>MATLKAQHLAKSYKGRQVVRDVSMSIDSGQIVGLLGPNGAGKTTCFYMIVGLVQADQGVVRIDEQNVTHLPMHGRARAGIGYLPQEASIFRKLSVSDNIMAILETRSDLDRNGRKEALEGLLQEFHIHHIRDNLGMSLSGGERRRVEIARALASAPKFILLDEPFAGVDPISVGDIKQIIHHLKAKGIGILITDHNVRETLDICETAYIVNDGQLIAEGDAESILANDLVKEVYLGHEFRLHHHHHH[2x];> MIVFRYLSREVLVTMSAVSAVLLVIIMSGRFIKYLAQAAQGLLDPGSLFLIMAFRIPGFLQLILPLGLFLGILLAYGRLYLESEMTVLSATGMSQKRLLGYTMAPALLVAILVAWLSLFLAPQGINQFALLLNKQDTLTEFDTLVPGRFQAMRDGTRVTYTEELSKDRGELAGIFISQKDLNSSNQERGISILVAEKGTQNIQADGSRYLILHNGYRYDGNPGQANYRAIQYDTYGVMLPKPEASSEVSERDAVPTADLFGSDNPRYQAELQWRLSTPLLVFVVTLLAVPLSRVNPRQGRFLKLLPAILLYMGYLALLIAVRGQLDKGKIPMAIGLWWVHGLFLAIGLLLFYWEPLRLKLAS;> MVKLDRYIGVTVFVAILAVLGVILGLALLFAFIDELNDISASYGIGDALRFIFLTAPRRAYDMLPMAALIGCLVGLGTLASNSELTIMRAAGVSLSRIVWAVMKPMLVLMLAGILVGEYVAPWTENIAQSGRALAQGGGDSQSSK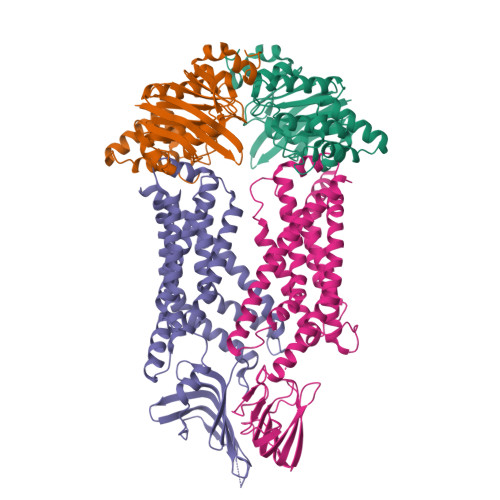RGLWHRQGREYIHINAVQPNGVLYGVTRYRFDEQRGLESASFAKRARFETDHWQLEEVTTTLLHPREKRSEVVKLPTERWDAQLSPQLLNTVVMEPEALSISGLWQYIHYLADQGLNNNRYWLAFWTKVLQPLVTAALVLMAISFIFGPLRSVTLGQRIFTGVLVGFVFRIAQDLLGPSSLVFDFPPLLAVVIPASICALAGVWLLRRAG> MMAGKSSLFKIILLGDG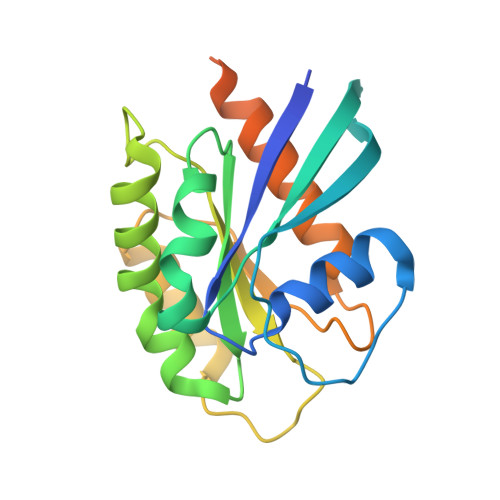GVGKSSLMNRYVTNKFDSQLFHTIGVEFLNKDLEVDGHFVTMQIWDTAGLERFRSLRTPFYRGSDCCLLTFSVDDSQSFQNLSNWKKEFIYYADVKEPESFPFVILGNKTDIKERQVSTEEAQAWCKDNGDYPYFETSAKDSTNVAAAFEEAVRRILATEDRSEHLIQTDTVNLHRKPKPNSSLEHHHHHH of transcription factors found in prokaryotes. N-terminal winged Helix Turn Helix (wHTH) DNA Binding Domain (DBD). two Rossmann fold-like sub domains (RD1, RD2). conformational changes which modify LTTR DNA binding sites promoter region DNA.

apo-DntR homotetramers adopt a compact homotetrameric configuration. well-defined electron density for the wHTH regions. apo-DntR they cannot bind salicylate and DntR cannot be activated. constraints in the crystal - packed closer to the tetrameric core. solution is different to that observed in the crystal. apo-DntR reported here result in very poor matches.

>MDLRDIDLNLLVVFNQLLLDRSVSTAGEKLGLTQPAVSNSLKRLRTALNDDLFLRTSKGMEPTPYALHLAEPVIYALNTLQTALTTRDSFDPFASTRTFNLAMTDIGEMYFMPPLMEALAQRAPHIQISTLRPNAGNLKEDMESGAVDLALGLLPELQTGFFQRRLFRHRYVCMFRKDHPSAKSPMSLKQFSELEHVGVVALNTGHGEVDGLLERAGIKRRMRLVVPHFIAIGPILHSTDLIATVPQRFAVRCEVPFGLTTSPHPAKLPDIAINLFWHAKYNRDPGNMWLRQLFVELFSEARHHHHHH[2x]> MWATLPLLCAGAWLLGVPVCGAAELCVNSLEKFHFKSWMSKHRKTYSTEEYHHRLQTFASNWRKINAHNNGNHTFKMALNQFSDMSFAEIKHKYLWSEPQNCSATKSNYLRGTGPYPPSVDWRKKGNFVSPVKNQGACGSCWTFSTTGALESAIAIATGKMLSLAEQQLVDCAQDFNNHGCQGGLPSQAFEYILYNKGIMGEDTYPYQGKDGYCKFQPGKAIGFVKDVANITIYDEEAMVEAVALYNPVSFAFEVTQDFMMYRTGIYSSTSCHKTPDKVNHAVLAVGYGEKNGIPYWIVKNSWGPQWGMNGYFLIERGKNMCGLAACASYPIPLV

Cathepsin H is a lysosomal cysteine protease of the papain superfamily involved in protein degradation. For preventing premature activation, cysteine proteases are synthesized as inactive proenzymes called zymogens that contain a prodomain and a mature (catalytic) domain, and the removal of the prodomain leads to the activation of the enzymes. Upon activation, cathepsin H displays a distinct proteolytic activity among the papain superfamily, functioning predominantly as an aminopeptidase that cleaves a single N-terminal residue from a polypeptide chain. Unique among papain-like cysteine proteases, the mini-chain (the octapeptide EPQNCSAT from the prodomain) remains bound to cathepsin H through a disulfide bond and is essential for the aminopeptidase activity.

Purified procathepsin H protein was not autoprocessed under the acidic crystallization condition and we were able to determine the crystal structure of procathepsin H at 2.00 Å resolution. Procathepsin H was well defined in the electron density map as a single polypeptide chain comprised of an N-terminal prodomain (Ala1P-Pro93P) and a C-terminal mature domain (Tyr1-Val220) with a disulfide bridge between Cys212 and the mini-chain Cys80P. bLigand/ion in the structure of procathepsin H: N-acetyl-D-glucosamine, β-D-mannopyranose, α-D-mannopyranose, sulfate ion, glycerol. Glycans could be assigned unambiguously in procathepsin H for the two glycosylation sites, Asn79P on the mini-chain of the prodomain and Asn115 on the mature domain. Cys26 is oxidized to S-oxy cysteine and adopts two alternative conformations in our crystal structure of procathepsin H. The oxidation may have happened during purification or crystallization as no reducing agent was present to preserve the formation of all disulfide bonds. The sidechain of His166 adopts an active orientation in procathepsin H with Nδ interacting with the sulfur of Cys26 at a distance of 3.1 Å and Nε interacting with Oδ of Asn186 at a distance of 2.8 Å, compared with cathepsin H where His166 was not involved in any interaction with Cys26 or Asn186 due to crystal packing. However, these three catalytic residues in procathepsin H are shielded by a group of hydrophobic residues Tyr72P, Leu73P, Trp74P from the prodomain, which effectively blocks the access to the catalytic Cys and prevents external substrates from entering the binding site. Structural comparison with cathepsin H revealed that the mini-chain in procathepsin H runs in the direction opposite to that of the substrates while the mini-chain in cathepsin H follows the substrate binding direction, suggesting that the negatively charged C-terminal carboxyl group in the mini-chain of cathepsin H is positioned to interact with the N-terminal amino group of the substrate whereas the cleaved mini-chain in procathepsin H needs to reorient to be involved in such interaction.>[2x]MLSHMVLTRQDIGRAASYYEDGADDYYAKDGDASEWQGKGAEELGLSGEVDSKRFRELLAGNIGEGHRIMRSATRQDSKERIGLDLTFSAPKSVSLQALVAGDAEIIKAHDRAVARTLEQAEAR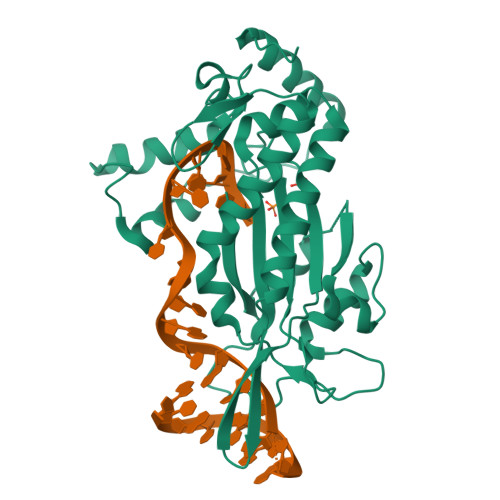AQARQKIQGKTRIETTGNLVIGKFRHETSRERDPQLHTHAVILNMTKRSDGQWRALKNDEIVKATRYLGAVYNAELAHELQKLGYQLRYGKDGNFDLAHIDRQQIEGFSKRTEQIAEWYAARGLDPNSVSLEQKQAAKVLSRAKKTSVDREALRAEWQATAKELGIDFS> GANDYVPSPITINTSTLPVVVIGPADAHTYPRVIGELTGTSNQYIFNGGSLIALMRGKFTPTLPKIGKITYNFRQGNNTQSSDFDIFDTGVPGLGIIIGMAGYWPATPLVPINSSSIYIDPVAANTNPNAYNGATGSFGARLYVAFVATGRLPNGYVTIPTKQLGHILLESNRASLNNKRLTAPVMLNGGRAHH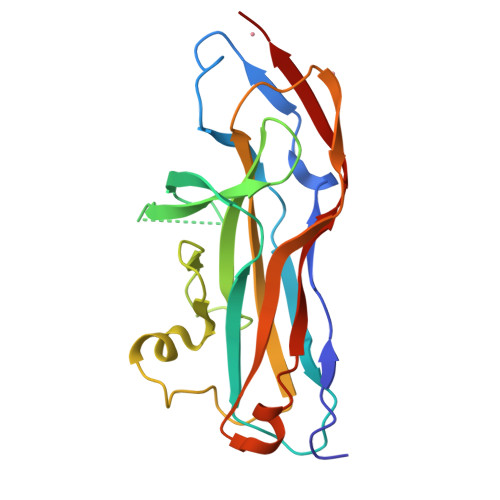HHHH> GSHMASPNGQTKPLPALKLALEYIVPAMNKHGICVVDDFLGKETGQQIGDEVRALHDTGKFTDGQLVSQKSDSSKDIRGDKITWIEGKEPGCETIGLLMSSMDDLICHCNGKLGSYKINGRTKAMVACYPGNGTGYVRHCDNPNGDGRCVTC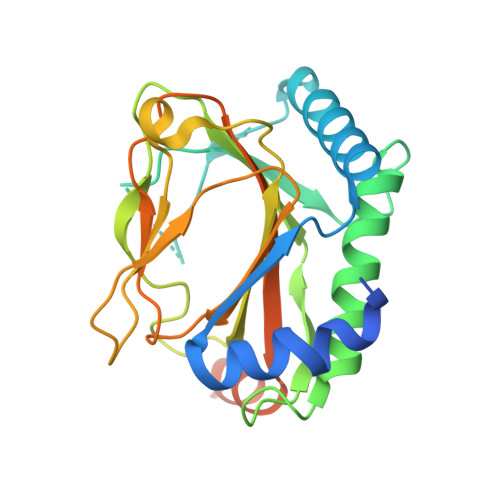IYYLNKDWDAKVSGGILRIFPEGKAQFADIEPKFDRLLFFWSDRRNPHEVQPAYATRYAITVWYFDADERAAAKVKYLTGEKGVRVELNKPSDSVGKDVF> MLAKRIIACLDVKDGRVVKGTNFENLRDSGDPVELGKFYSEIGIDELVFLDITAFVEKRKTMLELVEKVAEQIDIPFTVGGGIHDFETASELILRGADKVSINTAAVENPSLITQIAQTFGSQAVVVA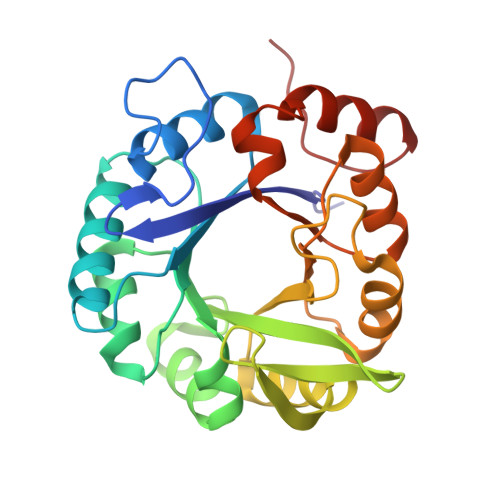IDAKRVDGEFMVFTYSGKKNTGILLRDWVVEVEKRGAGEILLTSIDRDGTKSGYDTEMIRFVRPLTTLPIIASGGAGKMEHFLEAFLAGADAALAASVFHFREIDVRELKEYLKKHGVNVRLEGL2-(4-DIMETHYLAMINOPHENYL)DIAZENYLBENZOIC 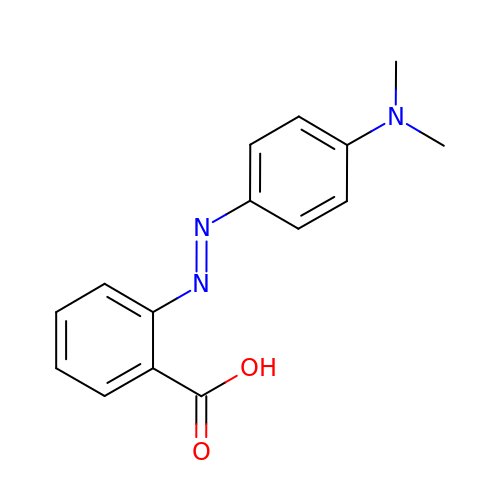ACID | C15 H15 N3 O2 | CEQFOVLGLXCDCX-WUKNDPDISA-N1,4-DIHYDROXY-5,8-BIS({2-[(2-HYDROXYETHYL)AMINO]ETHYL}AMINO)-9,10-ANTHRACENEDIONE | C22 H28 N4 O6 | 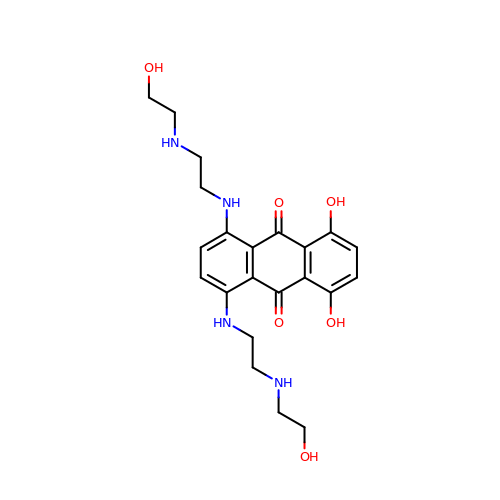KKZJGLLVHKMTCM-UHFFFAOYSA-N> MQGSWSVLKKNCSNFFPGLLAFAQQTQEAYGIWLRIYNRQQKYGPTDFVEQSETFSPDYHKRFHSQDKNMWVDKELCTEVSQKEVARLMTYKLDMWRMAHCAGALLATGGYAIPFGLFWLANDTWVPSSFNLTGEELRAWRE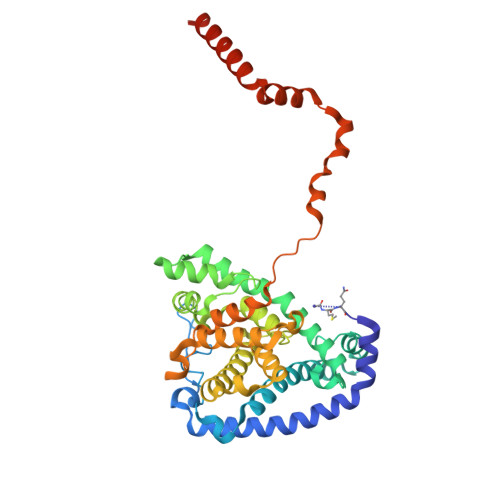AQDLYRYRSAPSYLTDTKWHFDFHAYPWNETQERAWDDLFEKNDVRRDPKVVRPAAEMYDGFIKFELIRRKSLRHLCRSMNIPTFPMLARLCNGTRVRDYWNLAWCEDYMVITQRLHESMTDEELYDYAWRRYLAPYDKNLNREQLMERVEDYFEFLGPDFVAHGKAPNLVILTNYVLGYYNDPAYLEGDISELDKNDYDHLASWGKDAFLRRLEFENGPLRDQVEAHTQRLLAERAAIAKGDNAAAVEGRHTA The class B MBLs are enzymes with the ability to hydrolyse virtually all β-lactam antibiotics, including carbapenems. Phylogenetically, MBLs can be grouped into three subclasses, B1 to B3.2 While enzymes belonging to subclasses B1 and B3 carry two Zn(II) binding sites (Zn1 and Zn2), B2 MBLs are mono-Zn(II) enzymes. In subclass B1, Zn1 is coordinated by three histidine residues (His/Gly116, His118 and His196), while the Zn2 binding site is coordinated by Asp120, Cys221 and His263.2,4–7 In B2 MBLs, the Zn1 binding site displays one altered residue (Asn116, His118 and His196), whereas the Zn2 site is identical to that of the subclass B1 MBLs. Here, we investigated three of these B1 MBLs,6 SHD-1, MYO-1 and ECV-1, in comparison with the clinically widespread enzyme NDM-1.

MYO-1 was encoded on a tet(X)-harbouring plasmid in Myroides odoratimimus, a widely distributed bacterium in natural environments. The structures of MYO-1 and ECV-1 were successfully solved by X-ray crystallography to 2.17 and 1.33 Å, respectively. For MYO-1 we found two molecules (chains A and B) in the asymmetrical unit with Rwork and Rfree of 0.22 and 0.25 (space group P65). Due to lack of electron density in chain B, the regions of N60 to K66, L93 to I96 and K104 to S105 could not be built. In contrast to the complex H-bond network in NDM-1 involving Ser69, Asp84, Lys121 and Ser262, we found different amino acids in MYO-1 (Cys69, Cys121, Gly262), ECV-1 (Cys69, Cys121, Gly262) and SHD-1 (Ala69, Arg121, Gly262). Compared with Arg121 (SHD-1) and Lys121 (NDM-1), we found a third cysteine (Cys121) within the active site of MYO-1 and ECV-1. These cysteines (Cys69, Cys121, Cys221) were in the vicinity of Asp120 (3–5 Å). The lack of Lys121 or Arg121 in MYO-1 and ECV-1 was compensated for by an extensive network of water molecules. Interestingly, this loop was shortened by one residue at position 231 in both MYO-1 and ECV-1. For MYO-1, the catalytic activity tended to be higher and its carbapenemase activity reached up to ∼70% to that of NDM-1.

>GQENKKEIINKPLTDSLIVYQTENLIINKLSNHIYEHISFLNTDDFGKVACNGMLVLNENKVVVFDTPTDDKSSLELINFVTNTLKSEIIGLIPTHFHDDCIGGITEFENHNIQTYVSKETIELLKDNGQEFSNPTKDFDNSLTLDIGNKKVYAEYFGEGHTKDNVVGYFPEDNAVFGGCLIKEIDASKGYLGDANIKEWSTTVEKVKLKYPNAKIVIPGHGKWGGIELFDYTIKLFE[2x]ethyl [2-(methylamino)-8-oxo-7,8-dihydro-1H-imidazo[4,5-g]quinazolin-6-yl]carbamate | C13 H14 N6 O3 | 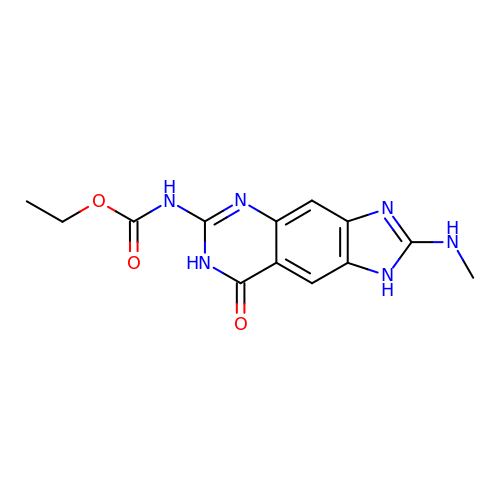KXOJIFFEGXMDQZ-UHFFFAOYSA-N TRPV6, a highly calcium-selective TRP channel, is overexpressed in endometrial cancers, leukemia, and carcinomas of the breast, prostate, colon, ovarian, and thyroid. TRPV6 has four subunits that form a transmembrane domain (TMD) with a central ion channel pore, an intracellular skirt domain enclosing a large cavity, and amphipathic TRP helices that run nearly parallel to the membrane and interact with both the TMD and the skirt. The TMD is composed of transmembrane helices S1–S6 and a re-entrant pore loop (P-loop) between S5 and S6. The first four transmembrane helices form a bundle to constitute the S1–S4 domain.

We used the TRPV6* construct that we developed earlier by modifying rat TRPV6 (rTRPV6) for crystallization. Importantly, in fluorimetric assays 2-APB inhibited calcium uptake through TRPV6* with a similar efficacy (IC50 = 156 ± 20 μM, n = 3) as in wild-type channels (IC50 = 184 ± 8 μM, n = 4). The TRPV6*2-APB structure does not exhibit substantial conformational rearrangements when compared to TRPV6* (the root mean square deviation, RMSD = 0.505). In each subunit of the TRPV6*2-APB tetramer, a pocket formed by the intracellular portions of the S1–S4 helices and the membrane-facing sides of the amphipathic TRP helices contained a strong density that matches the size and shape of 2-APB and was not observed in the TRPV6* structure. Notably, this binding pocket is distinct from the pocket at the S4–S5 interface that binds an activating lipid in TRPV641, agonists, such as resiniferatoxin (RTX) and capsaicin, and antagonists, such as capsazepine (CPZ), in TRPV142, and the inhibitor econazole in TRPV543. 2-APB binding is apparently mediated by multiple interactions. E402 in S2 appears to interact with the amino group of the 2-APB tail. In addition, the two phenyl rings of 2-APB are surrounded by the imidazole group of H425 in S3, the guanidinium group of R469 in S4, the hydrophobic side chains of Y466 in the S4–S5 linker, and M602 in the TRP domain. We have only been able to crystallize rat TRPV6 in the closed state, precluding a clear view of conformational changes associated with 2-APB-dependent inhibition.

> MGWSLPKEKGLILCLWNKFCRWFHRRESWAQSRDEQNLLQQKRIWESPLLLAAKENNVQALYKLLKFEGCEVHQKGAMGETALHIAALYDNNEAAQVLMEAAPELVFEPMTSELYEGQTALHIAVINQNVNLVRALLARGASVSARATGSVFHYRPHNLIYYGEHPLSFAACVGSEEIVRLLIEHGADIRAQDSLGNTVLHILILQPNKTFACQMYNLLLSYDGGDHLKSLELVPNNQGLTPFKLAGVEGNIVMFQHLMQKRKHIQWTYGPLTSTLYDLTEIDSSGDDQSLLELIVTTKKREARQILDQTPVKELVSLKWKRYGRPYFCVLGAIYVLYIICFTMCCVYRPLKPRITNRTNPRDNTLLQQKLLQEAYVTPKDDLRLVGELVSIVGAVIILLVEIPDIFRLGVTRFFGQTILGGPFHVIIVTYAFMVLVTMVMRLTNSDGEVVPMSFALVLGWCNVMYFARGFQMLGPFTIMIQKMIFGDLMRFCWLMAVVILGFASAFYIIFQTEDPDELGHFYDYPMALFSTFELFLTIIDGPANYDVDLPFMYSITYAAFAIIATLLMLNLLIAMMGDTHWRVAHERDELWRAQVVATTVMLERKLPRCLWPRSGICGREYGLGDRWFLRVEDRQDLNRQRIRRYAQAFQQQDDLYSEDLEKDSGEKLVPR>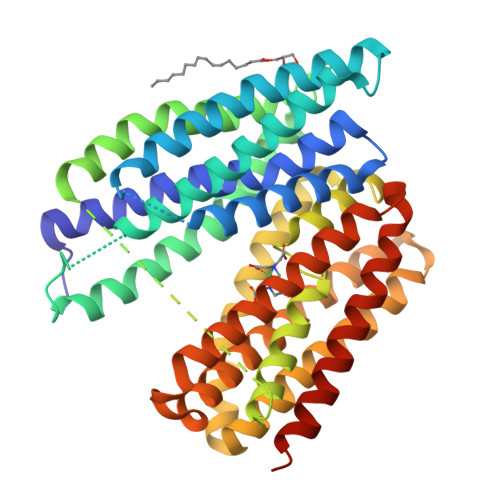 MKVQSLLRIETQLLLGRLLTRSGDQAWDFVVPFALLVIFPGKLQVAAFYYLIVKIGTFLLTPSSGKWIDTHPRIQVVKWGVWLQFFAILAGMVFFGMLDGLVRAGGRESWLLSVLFIALALSGVMASLGSQITDISVGNDLAPSLVAPEKLTHFNSWLRRIDLATEVGAPILAGALFAFHPEQLPLAGLFLIGLWNLVSFVPEYFLLRNVIQRSGLKIKVLTEAQSWKDTFHINLRGSFSDPIFWLILSYALLWLSVLSPHGVLLAAYLKDEMRLPETEIGLFRGLGAVFGLISTVSFPYLVRRLGLISSSRWHLGFQGVTLGIAVTAFAMGSTASVYVFLGCILLSRVGLYGFSNGEFELRQRLIPEGRRGELNSLSSLTTTSATLILFSAGSLLPQTEDFKYLVYVSLAAVLLANVVFIKWSSRQGVVTSGSENLYFQ We used de novo protein design to generate very closely related proteins that adopt two very different states—a short state and a long state, like a viral fusion protein—and then created a single molecule that can be found in both forms. Inspired by class I viral fusion proteins, such as influenza hemagglutinin, we chose homotrimeric helical bundles as the fundamental architecture. We decided on a design scheme with two divergent conformations containing a constant six-helix bundle “base” and a variable portion with three inner helices and three “flipping” helices. In the compact “short” state (∼66 Å height), the flipping helices fold back to interact with the inner helices; in the extended “long” state (∼100 Å height), they extend to form interactions with each other.

Crystal structures were determined for all potential bistable candidates (XAX_GGDQ, XXA_GVDQ, XAA_GGHN, and XAA_GVDQ), and we chose to focus on XAA_GVDQ because of the presence of a bound calcium. Detailed NMR and crystallographic characterizations of design XAA_GVDQ, described in the following paragraphs, suggest that this sequence may indeed populate both short and long states. In the absence of calcium, the 3D CM-CMHM NOESY and residual dipolar couplings (RDCs) were consistent with the short state. Because calcium-induced oligomerization or aggregation complicated NMR structure determination of the calcium-bound state, despite efforts to optimize pH, temperature, concentration, calcium, and buffer components, we turned to X-ray crystallography and sought to determine crystal structures in both the absence and presence of calcium. Most notably, the protein XAA_GVDQ adopts the designed short state by NMR in the absence of calcium, and the designed long state by crystallography in the presence of calcium.

>GSHMGDLKYSLERLREILERLEENPSEKQIVEAIRAIVENNAQIVEAIRAIVENNAQIVENNRAIIEALEAIGVDQKILEEMKKQLKDLKRSLERG[3x]>GAMGKIPNKQIKNKLLDDLKNLIETANEDRKKYEKKLEEEPSNQYGISIFKEIYWVASYETVADNTDRSKNYRKFTYATLNP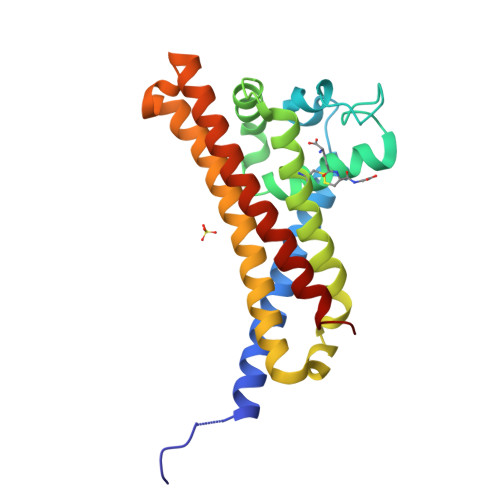INTNKLANLSKILIQSKQKTLLFGTFCNLGRTFDTAINHLYPKKDALDKLEISNLEKLKNSFEKLLSMKSIVSDMLNQLLLDYQDDKDSIKTDIAKLESHLTELYKQIEKKSSQATKLKNNILSISNL[2x]(2S)-2-aminobut-3-ynoic 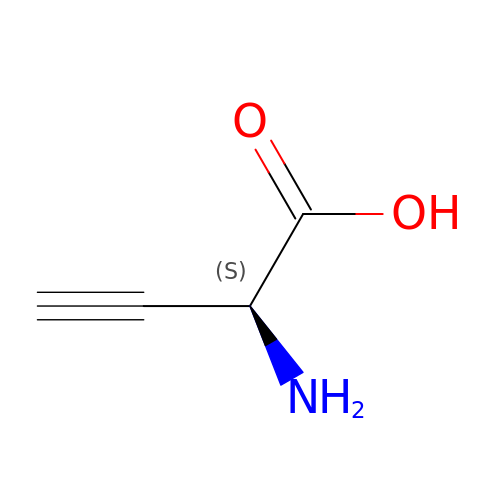acid | C4 H5 N O2 | DSUAJFIEKRKPEE-VKHMYHEASA-N>MNLPTAQEVQGLMARYIELVDVGDIEAIVQMYADDATVEDPFGQPPIHGREQIAAFFRQGLGGGKVRACLTGPVRASHNGCGAMPFRVEMVWNGQPCALDVIDVMRFDEH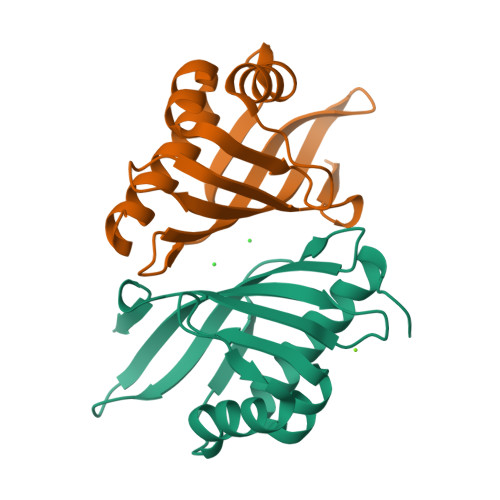GRIQTMQAYWSEVNLSVREPQ[2x]> GPMAWASSFDAFFKNFKRESKIISEYDITLIMTYIEENKLQKAVSVIEKVLRDIESAPLHIAVTGETGAGKSTFINTLRGVGHEEKGAAPTGAIETTMKRTPYPHPKLPNVTIWDLPGIGTTNFTPQNYLTEMKFGEYDFFIIISATRFKENDAQLAKAIAQMGMNFYFVRTKIDSDLDNEQKFKPKSFNKEEVLKNIKDYCSNHLQESLDSEPPVFLVSNVDISKYDFPKLETKLLQDLPAHKRHVFSLSLQSLTEATINYKRDSLKQKVFLEAMKAGALATIPLGGMISDILENLDETFNLYRSYFGLDDASLENIAQDLNMSVDDFKVHLRFPHLFAEHNDESLEDKLFKYIKHISSVTGGPVAAVTYYRMAYYLQNLFLDTAANDAIALLNSKALFEKKVGPYISEPPEYWEA

The p47 immunity-related GTPase (IRG) Irgb6 plays a pioneering role in host defense against Toxoplasma gondii infection. Irgb6 is recruited to the parasitophorous vacuole membrane (PVM) formed by T. gondii and disrupts it. The overall architectures of Irgb6 are similar to previously solved Irga6 or Irgb10 structures. They consist of an N-terminal helical domain (N-domain; amino acids 1–55; αA-αC) (purple in Fig 1A), a GTPase domain (G-domain; amino acids 56–239; H1-H5, αd, S1-S6) (green in Fig 1A), and a C-terminal helical domain (C-domain; amino acids 255–415; αF-αL) (pink in Fig 1A). The membrane-binding interface of Irgb6 assumes a unique conformation, composed of N- and C-terminal helical regions forming a phospholipid binding site.

The atomic structures of mouse Irgb6 monomer were solved in two states—with GTP and without nucleotide (nucleotide free: NF)—at 1.5 and 2.0 Å resolution, respectively. The NF structure did not have any nucleotide or ion in the pocket (NF Irgb6). The G1/P-loop (GxxxxGKS) in the GTP-bound state recognizes α- and β-phosphates of GTP, whereas that in the NF state override the corresponding binding site of the α- and β-phosphates, kicking the GDP out from the nucleotide-binding pocket of Irgb6. The G4 and following helices αd and H4 change their conformation largely from the NF state. The G-domain of NF Irgb6 exhibits a similar conformation to the NF form of Irga6, although the helix H4 and surrounding structures assume different conformations. This difference can be explained by the increased flexibility of G4 because of the absence of nucleotide, which is further stabilized by a neighboring molecule in the crystal packing environment. The helix H4 was stabilized by the interactions with the neighboring molecule. The αF-αGa loop was not visualized in the NF Irgb6 because of its high flexibility, whereas it was well defined in the GTP-bound Irgb6. The Irgb6 structures in two distinct nucleotide states take on similar conformations with overall root-mean square deviation (RMSD) of 2.4 Å. From the NF state to the GTP-bound state observed here, the conformational change of switch I pushes the αE toward the helical domains, generating rotational changes in the N- and C-domains.>MSDRFVIWAPSMHNEPAAKCGYCHGNKGGNMDQLFALDSWAHRYMNKMDVVKIENCTIGSFVEHMDVATYDRMCNMGFRRSGKFLYKVDPLRNCCRLYTIRTAPQELN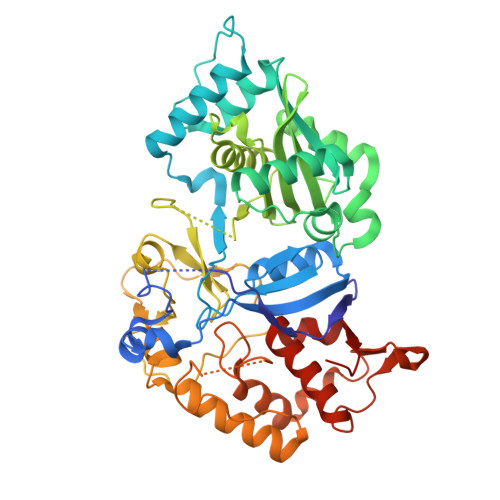MTKELKKCISRFATRITSEDYCPAAVASSDFVGKIVNAEMNSKTFYTRFEPALYSEEKYHLFVKYQEKVHQDYNNSPKSFKRFLCDTPFGPEAVLGTQESWEQLNNWQRMKPGEKLKHMGPVHECYYYEGKLIAITVSDILPSGISSVYFIWDPDYSKWSLGKLSALRDLAIIQRTNLQYYYLGYYIEDCPKMNYKANYGAEVLDVCHSKYIPLKPIQDMISRGKLFVIGKKKTKVTKELYLVDSETGRGEGFPTDNVVKYKNIAEEIYGVGGCAFKSANESALELKELYGIPYEEEDLDTIYHLKEHNGHAPNGIPNVVPGLLPLWELLDIMQSGKITDLEGRLFLFEIETEGIRPLINFYSEPPNVKKRICDVIRLFGFETCMKAVILYSEQMLEHHHHHH[12x]>MALRQCAIYGKGGIGKSTTTQNLVAALAEAGKKVMIVGCDPKADSTRLILHSKAQGTVMEMAASAGSVEDLELEDVLQIGFGGVKCVESGGPEPGVGCAGRGVITAINFLEEEGAYSDDLDFVFYDVLGDVVCGGFAMPIRENKAQEIYIVCSGEMMAMYAANNIAKGIVKYAHSGSVRLGGLICNSRKTDRED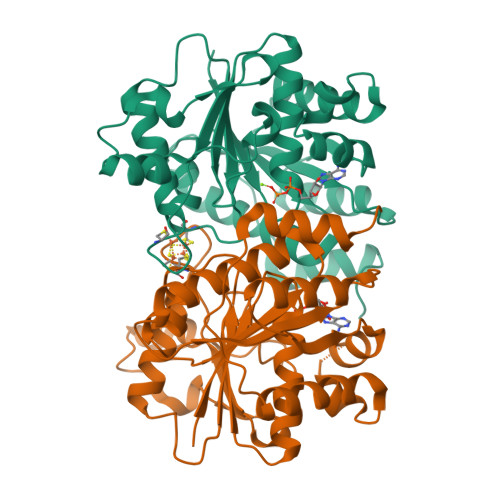ELIMALAAKIGTQMIHFVPRDNVVQHAEIRRMTVIEYDPKAGQADEYRALARKIVDNKLLVIPNPASMEELEELLMEFGIMEVEDESVVGKAAAEG[8x]> MVYVSNKYLTMSEMKVNAQYILNYLSSNGWTKQAICGMLGNMQSESTINPGLWQNLDEGNTSLGFGLVQWTPASNYINWANSQGLPYKNMDSELKRIIWEVNNNAQWINLR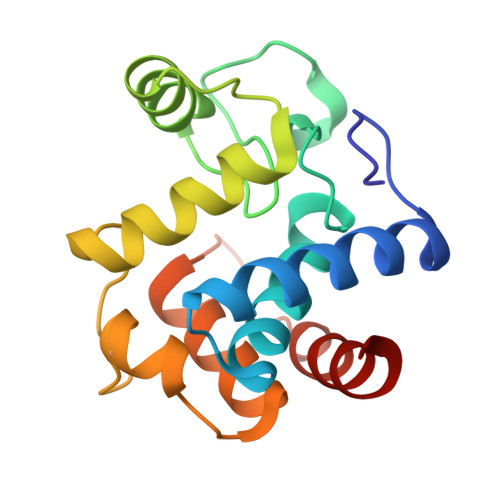DMTFKEYIKSTKTPRELAMIFLASYERPANPNQPERGDQAEYWYKNLS> MASAGVAAGRQAEDVLPPTSDQPLPDTKPLPPPQPPPVPAPQPQQSPAPRPQSPARAREEENYSFLPLVHNIIKCMDKDSPEVHQDLNALKSKFQEMRKLISTMPGIHLSPEQQQQQLQSLREQVR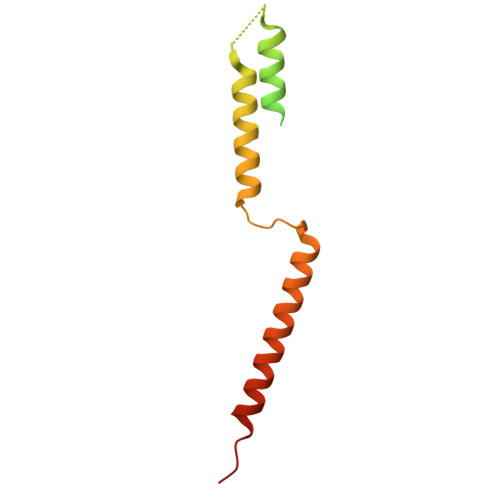TKNELLQKYKSLCMFEIPKE> SAGATAADGPCALRELSVDLRAERSVLIPETYQANNCQGVCGWPQSDRNPRYGNHVVLLLKMQARGAALARPPCCVPTAYAGKLLISLSEERISAHHVPNMVATECGCR;> GPHMPPNRRTCVFFEAPGVRGSTKTLGELLDTGTELPRAIRCLYSRCCFGIWNLTQDRAQVEMQGCRDSDEPGCESLHCDPSPRAHPS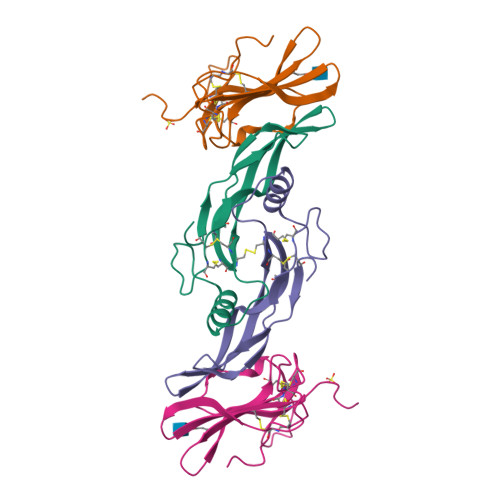PGSTLFTCSCGTDFCNANYSHLP> KELVLALYDYQEKSPDEVTMKKGDILTLLN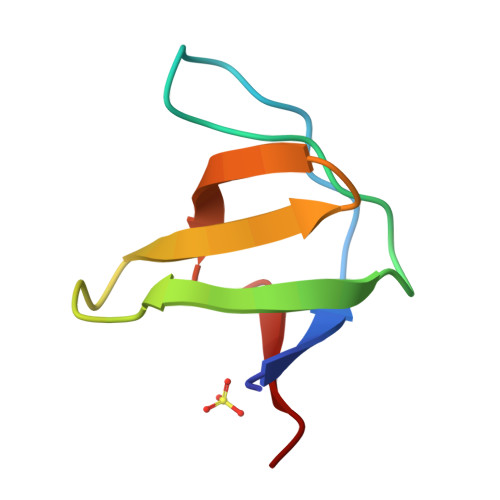STNKDWWKVEVNDRQGFVPAAYVKKLD>QFTERALTILTLAQKLASDHQHPQLQPIHILAAFIETPEDG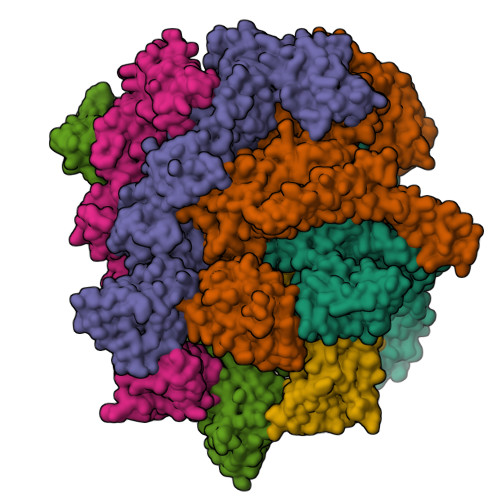SVPYLQNLIEKGRYDYDLFKKVVNRNLVRIPQQQPAPAEITPSYALGKVLQDAAKIQKQQKDSFIAQDHILFALFNDSSIQQIFKEAQVDIEAIKQQALELRGNTRIDSRGADTNTPLEYLSKYAIDMTEQARQGKLDPVIGREEEIRSTIRVLARRIKSNPCLIGEPGIGKTAIIEGVAQRIIDDDVPTILQGAKLFSLDLAALTAGAKYKGDFEERFKGVLKEIEESKTLIVLFIDEIHMLMGNGKDDAANILKPALSRGQLKVIGATTNNEYRSIVEKDGAFERRFQKIEVAEPSVRQTVAILRGLQPKYEIHHGVRILDSALVTAAQLAKRYLPYRRLPDSALDLVDISCAGVAVARDSKPEELDSKERQLQLIQVEIKALERDEDADSTTKDRLKLARQKEASLQEELEPLRQRYNEEKHGHEELTQAKKKLDELENKALDAERRYDTATAADLRYFAIPDIKKQIEKLEDQVAEEERRAGANSMIQNVVDSDTISETAARLTGIPVKKLSESENEKLIHMERDLSSEVVGQMDAIKAVSNAVRLSRSGLANPRQPASFLFLGLSGSGKTELAKKVAGFLFNDEDMMIRVDCSELSEKYAVSKLLGTTAGYVGYDEGGFLTNQLQYKPYSVLLFDEVEKAHPDVLTVMLQMLDDGRITSGQGKTIDCSNCIVIMTSNLGAEFINSQQGSKIQESTKNLVMGAVRQHFRPEFLNRISSIVIFNKLSRKAIHKIVDIRLKEIEERFEQNDKHYKLNLTQEAKDFLAKYGYSDDMGARPLNRLIQNEILNKLALRILKNEIKDKETVNVVLKKGKSRDENVPEEAEECLEVLPNHE[6x]>GNKEKADQQKAVTDIVALENALDMYKLDNSVYPTTDQGLEALVTKPTNPEPRNYREGGYIKRLPKDPWGNDYQYLSPGDKGTIDVFTLGADGQEGGEGTGADIGNWNIQDFQLE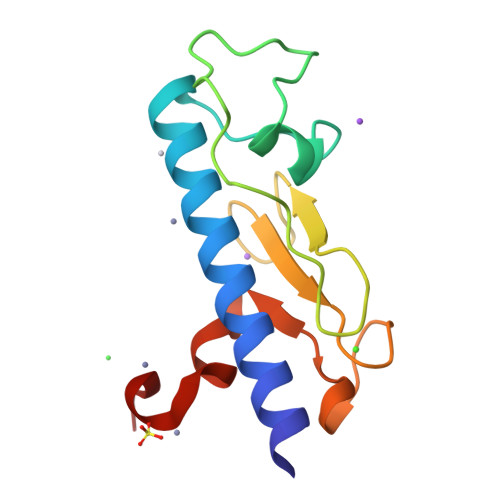HHHHHH[12x]Several transcription factors of the Rrf2 family use an iron-sulfur cluster to regulate DNA binding through effectors such as nitric oxide (NO), cellular redox status and iron levels. [4Fe-4S]-NsrR from Streptomyces coelicolor (ScNsrR) modulates expression of three different genes via reaction and complex formation with variable amounts of NO, which results in detoxification of this gas. The principal regulatory target of this TF is, in most organisms, the hmp gene, which encodes a flavohemoglobin that converts NO to nitrate (NO3−) or nitrous oxide (N2O) under aerobic or anaerobic conditions, respectively. Tightest binding was observed for hmpA1, followed by nsrR and hmpA2.25 In the presence of NO, the ScNsrR [4Fe-4S] cluster is rapidly lost, causing the dissociation of the protein-DNA complex.

Here, we report the 3.0 Å resolution X-ray structure of ScNsrR complexed with a 23-bp hmpA1 operator fragment and use it, alongside the structures referred to above, to establish what determines the DNA binding specificity among the three structurally-related iron-sulfur Rrf2 family proteins IscR, RsrR and NsrR. The 23 bp hmpA1 operator fragment has a B-DNA conformation. The double helix runs almost straight through the central 11 bp region and bends at its extremes around α-helix 3 of each of the NsrR subunits. The distance between phosphate P atoms across the minor groove (MiG) decreases from 12.6 Å at the center of the fragment to 9.6 Å between nucleotides 0 and + 4 of the other strand. Minimal MiG distances are observed for the + 4 and −7 phosphates, which respectively interact with the His42 and His52 imidazole groups. Most of the ScNsrR contacts are made with the phosphate backbone of the hmpA1 operator. The His42-Nδ1 and His52-Nε2 atoms interact with the respective 5’-phosphate groups of nucleotides +4 and −7 in opposite strands. There are only a few specific interactions between ScNsrR amino acid side chains and the nucleobases of the hmpA1 operator. The 58–61 and 66 wing residues bind edge-on to the MiG, with Arg60 making the most contacts to the DNA. There are few structural changes in [4Fe-4S]-ScNsrR upon its binding to the hmpA1 operator.

>MRLTKFTDLALRSLMRLAVVRDGDEPLATREVAEVVGVPYTHAAKAITRLQHLGVVEARRGRGGGLTLTDLGRRVSVGWLVRELEGEAEVVDCEGDNPCPLRGACRLRRALRDAQEAFYAALDPLTVTDLVAAPTGPVLLGLTDRPSGKLAAALEHHHHHH[2x]> SGTTNTVAAYNLTWKSTNFKTILEWEPKPVNQVYTVQISTKSGDWKSKCFYTTDTECDLTDEIVKDVKQTYLARVFSYPAGNVESTGSAGEPLYENSPEFTPYLETNLGQPTIQSFEQVGTKV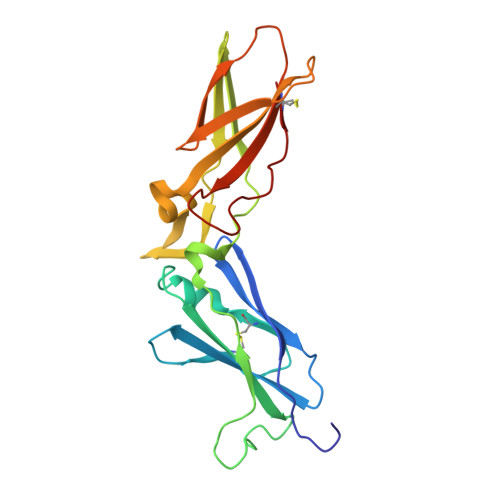NVTVEDERTLVRRNNTFLSLRDVFGKDLIYTLYYWKSSSSGKKTAKTNTNEFLIDVDKGENYCFSVQAVIPSRTVNRKSTDSPVECM>[2x]SELNEKLATAWEGFTKGDWQNEVNVRDFIQKNYTPYEGDESFLAGATEATTTLWDKVMEGVKLENRTHAPVDFDTAVASTITSHDAGYINKQLEKIVGLQTEAPLKRALIPFGGIKMIEGSCKAYNRELDPMIKKIFTEYRKTHNQGVFDVYTPDILRCRKSGVLTGLPDAYGRGRIIGDYRRVALYGIDYLMKDKLAQFTSLQADLENGVNLEQTIRLREEIAEQHRALGQMKEMAAKYGYDISGPATNAQEAIQWTYFGYLAAVKSQNGAAMSFGRTSTFLDVYIERDLKAGKITEQEAQEMVDHLVMKLRMVRFLRTPEYDELFSGDPIWATESIGGMGLDGRTLVTKNSFRFLNTLYT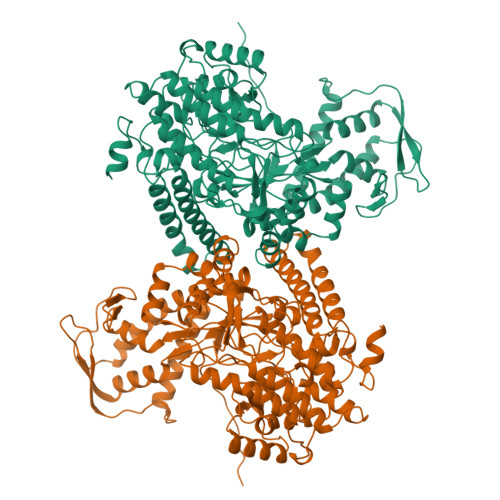MGPSPEPNMTILWSEKLPLNFKKFAAKVSIDTSSLQYENDDLMRPDFNNDDYAIACCVSPMIVGKQMQFFGARANLAKTMLYAINGGVDEKLKMQVGPKSEPIKGDVLNYDEVMERMDHFMDWLAKQYITALNIIHYMHDKYSYEASLMALHDRDVIRTMACGIAGLSVAADSLSAIKYAKVKPIRDEDGLAIDFEIEGEYPQFGNNDPRVDDLAVDLVERFMKKIQKLHTYRDAIPTQSVLTITSNVVYGKKTGNTPDGRR> MVQELSIERLLEMESLVADPSEEFQFLRVGPDSNVPPKFRAPVSSLCQIGNKQIAALVVWARDIPHFSQLEMEDQILLIKGSWNELLLFAIAWRSMEFLTEERDGVDGTGNRTTSPPQLMCLMPGMTLHRNSALQAGVGQIFDRVLSELSLKMRTLRVDQAEYVALKAIILLNPDVKGLKNRQEVEVLREKMFLCLDEYCRRSRSSEEGRFAALLLRLPALRSISLKSFEHLFFFHLVADTSIAGYIRDALRNHAPPIDTNMM;> GSHMASMTGGQQMGRDPLKNVPPLTANQKSLIARLVYYQEGYEQPSEEDLKRVTQTWQSDEDDEDS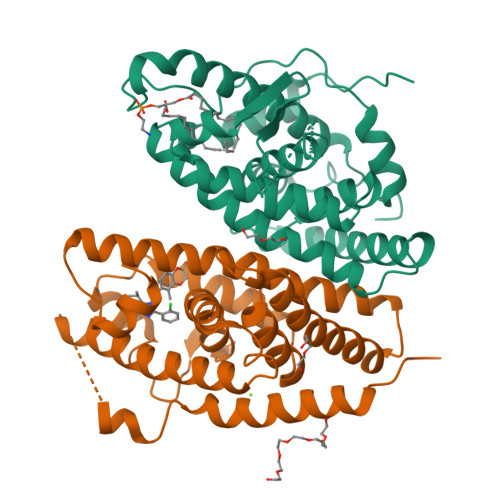DMPFRQITEMTILTVQLIVEFAKGLPGFSKISQSDQITLLKACSSEVMMLRVARRYDAATDSVLFANNQAYTRDNYRKAGMAYVIEDLLHFCRCMYSMMMDNVHYALLTAIVIFSDRPGLEQPSLVEEIQRYYLNTLRVYILNQNSASPRSAVIFGKILGILTEIRTLGMQNSNMCISLKLKNRKLPPFLEEIWDVADVA> MSGDYRITLEELRYISVFHSITGVTAYRCIVDEENNRLIFLVSEGEAGRAIGRGGRLIK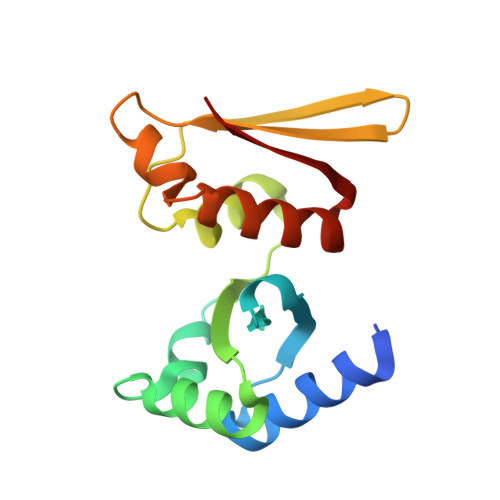LLREALGKNIEVVEYSSDLERIVKNLFPGVKIESINVRERNGVKQVVIKVSEDDKGAAIGKGGKNVKRARLVLSKLFGVEKVVIR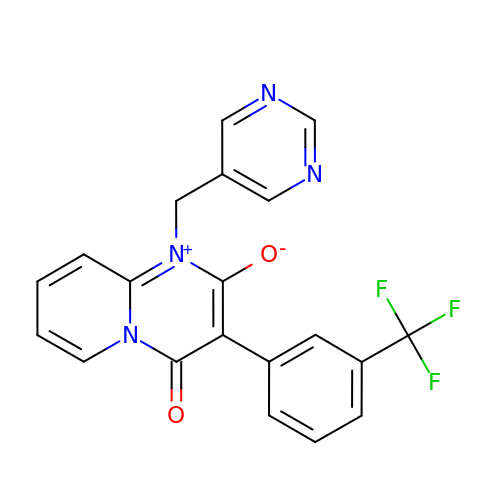4-oxidanylidene-1-(pyrimidin-5-ylmethyl)-3-[3-(trifluoromethyl)phenyl]pyrido[1,2-a]pyrimidin-1-ium-2-olate | C20 H13 F3 N4 O2 | LHZOTJOOBRODLL-UHFFFAOYSA-N>MHVKERYKNFLNQHVGPDMSVQRCNSEIGPNNRKITLSGTDNGCKPVNTFILANKRLIKTVCGRAGSPQGNMVRSNQPFPVVKCVLNNGERHPYCEYRGTRSTRYIVL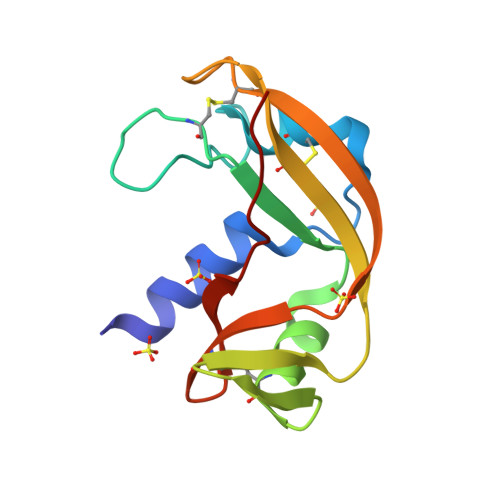KCEEGWPVHYHEDEVNVG[2x]> MGRQIPPDPVFGDVLVAKLINRVMWD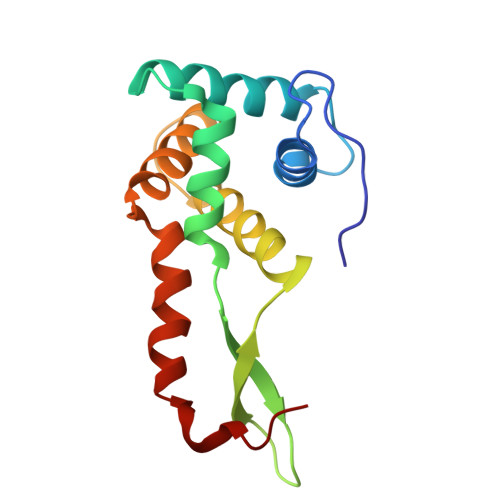GKKTIAQKIVYGAFDIIREKTKKDPLEVFRQAVENVKPVLEVRPRRVGGATYQVPIEVQEPRRTSLALRWIVEAARAKKGRPMKEKLAEEIIAAYNNTGTAIKKKEDTHRMAEANRAFAHYRW> GSHMGLFNAHAVAQQRADRIATLLQSFADGQLDTAVGEAPAPGYERHYDSLRALQRQLREQRAELQQVESLEAGLAEMSRQHEAGWIDQTIPAERLEGRAARIAKGVNELVAAHIAVKMKVVSVVTAYGQGNFEPLMDRLPGKKAQITEAIDGVRERLRGAAE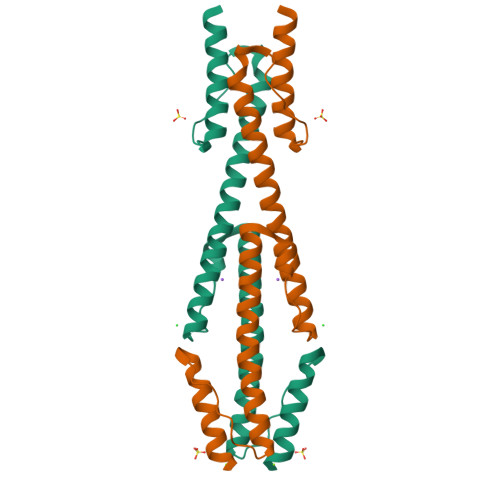ATSAQLATAAYN> SSQIRQNYSTEVEAAVNRLVNLYLRASYTYLSLGFYFDRDDVALEGVCAFFRELAEEKREGAERLLKMQNQRGGRALFQDLQKPSQDEWGT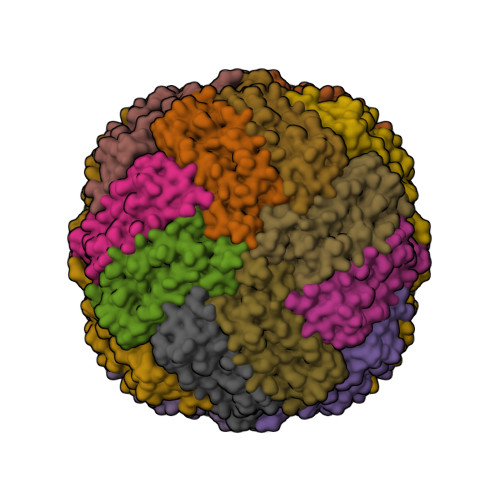TPDAMKAAIVLEKSLNQALLDLHALGSAQADPHLCDFLESHFLDEEVKLIKKMGDHLTNIQRLVGSQAGLGEYLFERLTLKHD> GRNQKPSRLTRSANNVLLEKGPTVERSTRMSNPWKAFMEKYDIERTHSSGVRVDLGEDAEVENAKYRIPAGRCPVFGKGIVIENSAVSFLKPVATGDQRLKDGGFAFPNANDHISPMTLENLKARYKDNVEMMKLNDIALCRTHAASFVMAGDQNSNYRHPAVYDEKEKTCHMLYLSAQENMGPRYCSPDAQNRDAVFCFKPDKDESFENLVYLSKNVRNDWDKKCPRKNLGNAKFGLWVDGNCEEIPYVKEVEAKDLRECNRIVFEASASDQPTQYEEEMTDYQKIQQGFRQNNREMIKSAFLPVGAFNSDNFKSKGRGFNWANFDSVKKKCYIFNTKPTCLIN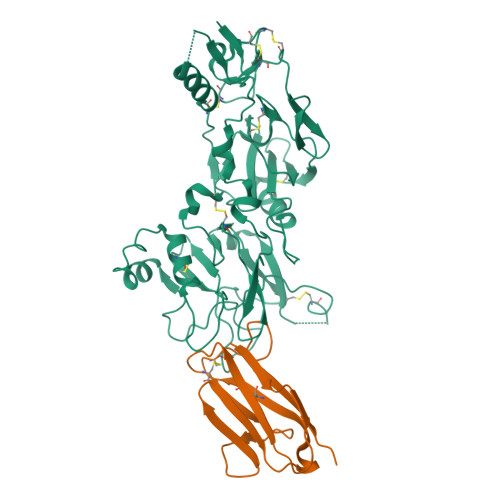DKNFIATTALSHPREVDLEFPCSIYKDEIEREIKKQSRNMNLYSVDGERIVLPRIFISNDKESIKCPCEPEHISQSTCNFYVCNCVEKRAEIKENNQVVIKEEFRDYYENGEEKSNKQGS;> LQVDIVPSQGEISVGESKFFLCQVAGMLPTCEISWFSPNGEKLTPNQQRISVVWNDDSSTLTIYNANIDDAGIYKCVVHGPQCPRLTWSLGLPEATVNVKIFQGGGGSEQKLISEEDLSGENLYFQ>[2x]GSPEF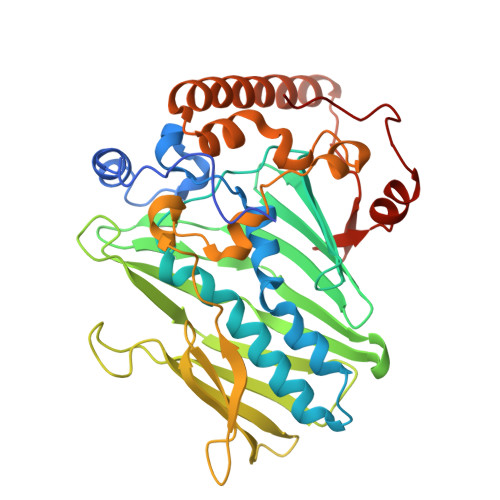SGREAKSRRRTSLPAPSPSSSNISLWNILRNNIGKDLSKVAMPVELNEPLNTLQRLCEELEYSELLDKAAQIPSPLERMVYVAAFAISAYASSYYRAGSKPFNPVLGETYECIREDKGFQFFSEQVSHHPPISACHAESRNFVFWQDVRWKNKFWGKSMEIVPIGTTHVTLPVFGDHFEWNKVTSCIHNILSGQRWIEHYGEIVIKNLHDDSCYCKVNFIKAKYWSTNAHEIEGTVFDRSGKAVHRLFGKWHESIYCGGGSSSACVWRANPMPKGYEQYYSFTQFALELNEMDPSSKSLLPPTDTRFRPDQRFLEEGNLEEAEIQKQRIEQLQRERRRVLEENHVEHQPRFFRKSDGSWVSNGTYLELRKDLGFSKLDHPVLW> KQQLTEDGDSFLHLAIIHEEKALTMEVIRQVKGDLAFLNFQNNLQQTPLHLAVITNQPEIAEALLGAGCDPELRDFRGNTPLHLACEQ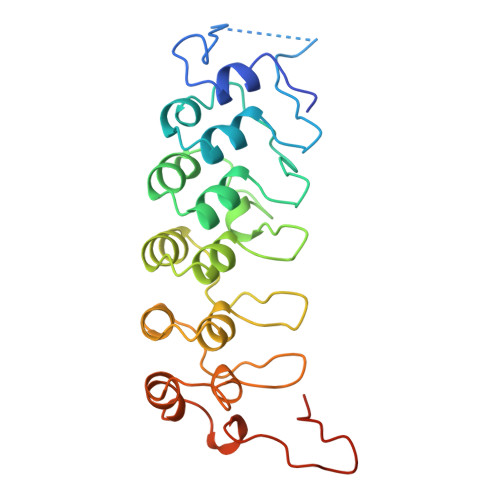GCLASVGVLTQSCTTPHLHSILKATNYNGHTCLHLASIHGYLGIVELLVSLGADVNAQEPCNGRTALHLAVDLQNPDLVSLLLKCGADVNRVTYQGYSPYQLTWGRPSTRIQQQLGQLTLENLQMLPESEDEESYDTESEFTEFTEDE N-PROPYL-TARTRAMIC ACID | C7 H13 N O5 | 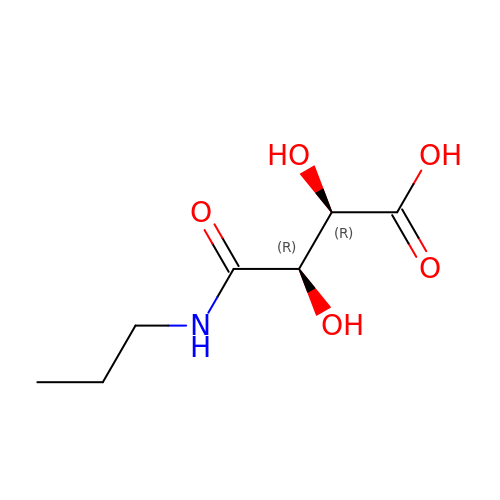LNEZKQHJUNIZIS-RFZPGFLSSA-N> GPMVAMFQEDNGTSSVASSPLQVFSTMSLNRPTLLASSSPFHCLKDLKPEERGLYLIHLLLTCANHVASGSLQNANAALEQLSHLASPDGDTMQRIAAYFTEALANRILKSWPGLYKALNATQTRTNNVSEEIHVRRLFFEMFPILKVSYLLTNRAILEAMEGEK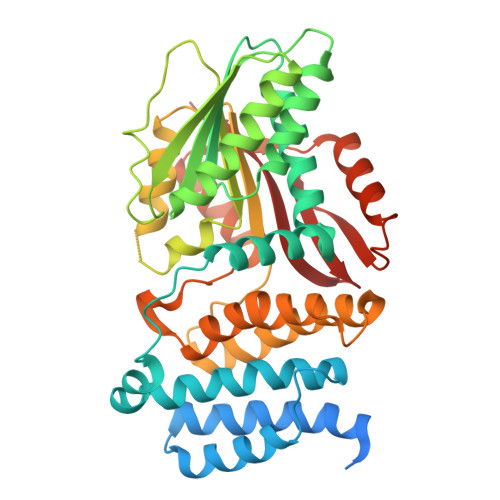MVHVIDLDASEPAQWLALLQAFNSRPEGPPHLRITGVHHQKEVLEQMAHRLIEEAEKLDIPFQFNPVVSRLDCLNVEQLRVKTGEALAVSSVLQLHTFLASDDDLMENDMSNNNGYSPSGDSASSLPLPSSGRTDSFLNAIWGLSPKVMVVTEQDSDHNGSTLMERLLESLYTYAALFDCLETKVPRTSQDRIKVEKMLFGEEIKNIISCEGFERRERHEKLEKWSQRIDLAGFGNVPLSYYAMLQARRLLQGCGFDGYRIKEESGCAVICWQDRPLYSVSAWRCRK> GYEEREGGFRKETVERLLRLHFRDGRTRVNGDALLLMAELLKVFVREAAARAARQAQA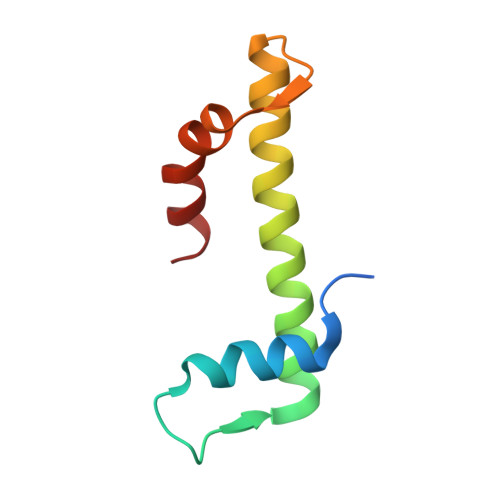EDLEKVDIEHVEKVLPQLLLDFV>MAKKIITVNVNGKAQEKAVEPRTLLIHFLREELNLTGAHIGCETSHCGACTVDIDGRSVKSCTHLAVQCDGSEVLTVEGLANKGVLHAVQEGFYKEHGLQCGFCTPGMLMRAYRFLQENPNPTEAEIRMGMTGNLCRCTGYQNIVKAVQYAARKLQEPSTAAA[2x];>[2x]MNAPVQDAEARELALAGMGASRLRKEDARFIQGKGNYVDDIKMPGMLHMDIVRAPIAHGRIKKIHKDAALAMPGVHAVLTAEDLKPLKLHWMPTLAGDVAAVLADEKVHFQMQEVAIVIADDRYIAADAVEAVKVEYDELPVVIDPIDALKPDAPVLREDLAGKTSGAHGPREHHNHIFTWGAGDKAATDAVFANAPVTVSQHMYYPRVHPCPLETCGCVASFDPIKGDLTTYITSQAPHVVRTVVSMLSGIPESKVRIVSPDIGGGFGNKVGIYPGYVCAIVASIVLGRPVKWVEDRVENISTTAFARDYHMDGELAATPDGKILGLRVNVVADHGAFDACADPTKFP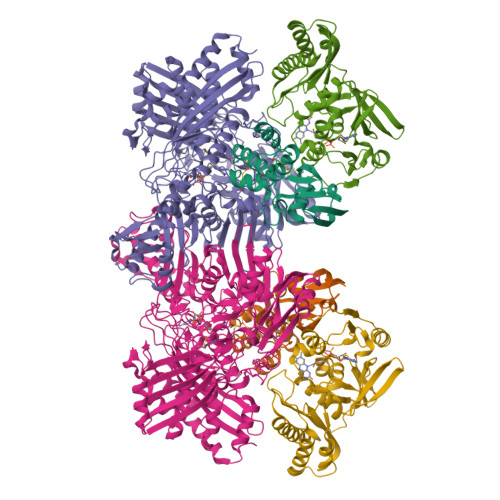AGLFHICSGSYDIPRAHCSVKGVYTNKAPGGVAYRCSFRVTEAVYLIERMVDVLAQKLNMDKAEIRAKNFIRKEQFPYTTQFGFEYDSGDYHTALKKVLDAVDYPALRAEQAARRADPNSPTLMGIGLVTFTEVVGAGPSKMCDILGVGMFDSCEIRIHPTGSAIARMGTITQGQGHQTTYAQIIATELGIPSEVIQVEEGDTSTAPYGLGTYGSRSTPVAGAAIALAARKIHAKARKIAAHMLEVNENDLDWEVDRFKVKGDDSKFKTMADIAWQAYHQPPAGLEPGLEAVHYYDPPNFTYPFGIYLCVVDIDRATGETKVRRFYALDDCGTRINPMIIEGQIHGGLTEGYAVAMGQQMPFDAQGNLLGNTLMDYFLPTAVETPHWETDHTVTPSPHHPIGAKGVAESPHVGSIPTFTAAVVDAFAHVGVTHLDMPHTSYRVWKSLKEHNLAL;>MIPPRFEYHAPKSVGEAVALLGQLGSDAKLLAGGHSLLPMMKLRFAQPEHLIDINRIPELRGIREEGSTVVIGAMTVENDLISSPIVQARLPLLAEAAKLIADPQVRNRGTIGGDIAHGDPGNDHPALSIAVEAHFVLEGPNGRRTVPADGFFLGTYMTLLEENEVMVEIRVPAFAQGTGWAYEKLKRKTGDWATAGCAVVMRKSGNTVSHIRIALTNVAPTALRAEAAEAALLGKAFTKEAVQAAADAAIAICEPAEDLRGDADYKTAMAGQMVKRALNAAWARCA[2x]> MDSPVLQSAYDPSGQYLCYVTVALDKQRVGVQ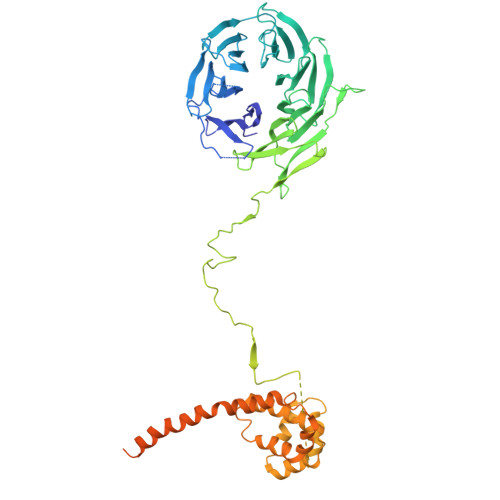PTQRATSSGVDTVWNENFLYLEDSKLKVTCLKWVNLASSDTVAIILGMNNGEIWLYSVLANEVTYKFTTGNSYEIKDIDLMGNQLWCIDSSDAFYQFDLLQFKLLQHFRINNCVQLNKLTIVPAGDSVAQLLVASHSISLIDIEEKKVVMTFPGHVSPVSTLQVITNEFFISGAEGDRFLNVYDIHSGMTKCVLVAESDIKELSHSGQADSIAVTTEDGSLEIFVDPLVSSSTKKRGNKSKKSSKKIQIVSKDGRKVPIYNAFINKDLLNVSWLQNATMPYFKNLQWREIPNEYTVEISLNWNNKNKSADRDLHGKDLASATNYVEGNARVTSGDNFKHVDDAIKSWERELTSLEQEQAKPPQANELLTETFGDKLESSTVARISGKKTNLKGSNLKTATTTGTVTVILSQALQSNDHSLLETVLNNRDERVIRDTIFRLKPALAVILLERLAERIARQTHRQGPLNVWVKWCLIIHGGYLVSIPNLMSTLSSLHSTLKRRSDLLPRLLALDARLDCTINKFKTLNYEAGDIHSSEPVVEEDEDDVEYNEELDDAGLIEDGEESYGSEEEEEGDSDNEEEQKHTSSKQDGRLETEQSDGEEEAGYSDVEME>[4x]MYKDLEGKVVVITGSSTGLGKSMAIRFATEKAKVVVNYRSKEDEANSVLEEIKKVGGEAIAVKGDVTVESDVINLVQSAIKEFGKLDVMINNAGLENPVSSHEMSLSDWNKVIDTNLTGAFLGSREAIKYFVENDIKGTVINMSSVHEKIPWPLFVHYAASKGGMKLMTETLALEYA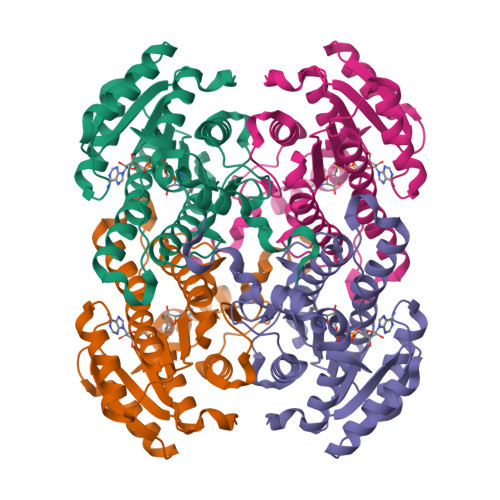PKGIRVNNIGPGAINTPINAEKFADPEQRADVESMIPMGYIGEPEEIAAVAAWLASSEASYVTGITLFADGGMTQYPSFQAGRG> MRDNSDTVKMKRGINIGNALESPKDFPWDVKMSNKFFDDIKDAGFDTVRIPVRFSDYTSDSDNFKIDEDFFKKIDKYVDYALDKDLIVVLDLHHFEEIMKEPRVHKEKFLKIWQQIANRYQKYDKKLVFELLNEPKENLYSQLLNEYIEEAIKIIRKTNPKRTIIVGPYNFYQIDYLNELNIPKDSNIVVSFHYYEPNDFAFQGNIYHKGFEHLSNITWEGTNEQMDYLKKRFDTVENWANKNNVKIFLGEFGVTKEAPETSRRAWVKAVREEAEKRNFSWAYWELASGFGIYNQIEGTWDRDILSALIEKRLEHHHHHH

Our subsequent analysis of the cognate glycosyl hydrolase, CcsZ, reveals the Clostridial cellulose synthase contains a functionally analogous, but structurally distinct, glycosyl hydrolase from the known Gram-negative cognate glycosyl hydrolase BcsZ. In agreement with typical GH-5 enzymes, CcsZ folds into an overall structure adopting a distorted TIM barrel fold, in which an (α/β)8 barrel is formed at the core of the fold by eight parallel β-strands. The extended C-terminal loops shape a deep cleft that is typical of GH-5, where both the active site and the cleft for substrate accommodation are located. The GH-5 consensus catalytic acid/base and nucleophile residues are present in CcsZ as Glu-164 and Glu-281, respectively.

We engineered and synthesized the soluble domain of ccsZ from C. difficile, corresponding to residues 30–340 of the GenPept entry WP_077724661.1, into the pET21 expression vector to generate a recombinant His-tagged expression construct of CcsZ. Our CcsZ crystals grew in space group P 21 and diffracted X-rays well to 1.75 Å resolution with a single copy of CcsZ in the asymmetric unit. Model building and subsequent refinement resulted in an improved Rwork and Rfree of 0.227 and 0.260, respectively. The model covers almost the entirety of the CcsZ construct, from residues 38 to 337 in the sequence, although residue Ser91 could not be reliably built into the model due to a lack of electron density. Interestingly, we observed this groove to be strongly negatively charged in CcsZ, which is not a typical feature of GH-5. Our structure of apo-CcsZ superimposed excellently on apo-TmCel5A, with a root mean square deviation (r.m.s.d.) of 0.677 Å across 252 equivalent Cα atoms, as expected given the reasonably high sequence identity (43%) between these proteins and the highly conserved GH-5 fold. The TmCel5A-cellotetraose complex also superimposed well over CcsZ, with an r.m.s.d. of 0.620 Å over 242 equivalent Cα atoms. A comparison of the substrate-binding cleft, informed by the positioning of the cellotetraose ligand of TmCel5A, demonstrated a clear difference between the subsite architectures of the two enzymes. The residues that contribute to the -1 and -2 subsites of TmCel5A appear to be partially conserved in CcsZ, present as H123, H124, N163, Y225 and N48.> MEDTQM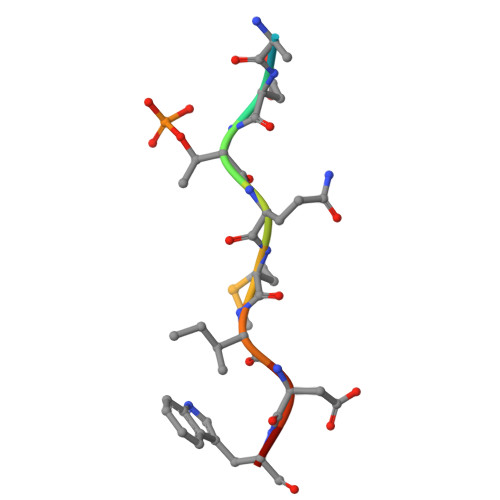IDWD>MANELTWHDVLAEEKQQPYFLNTLQTVASERQSGVTIYPPQKDVFNAFRFTELGDVKVVILGQDPYHGPGQAHGLAFSVRPGIAIPPSLLNMYKELENTIPGFTRPNHGYLESWARQGVLLLNTVLTVRAGQAHSHASLGWETFTDKVISLINQHREGVVFLLWGSHAQKKGAIIDKQRHHVLKAPD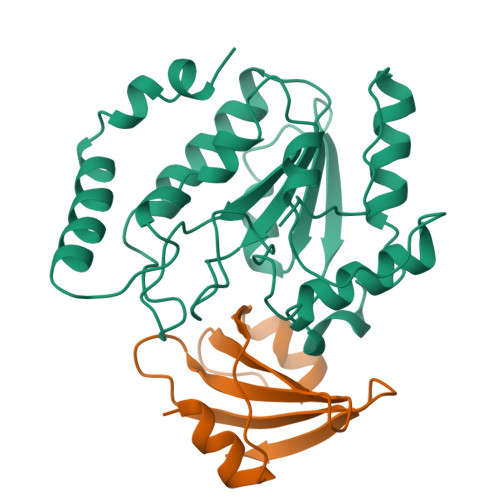PSPLSAHRGFFGCNHFVLANQWLEQRGETPIDWMPVLPAESE[2x];>MTNLSDIIEKETGKQLVIQESILMLPEEVEEVIGNKPESDILVHTAYDESTDENVMLLTSDAPEYKPWALVIQDSNGENKIKML[2x]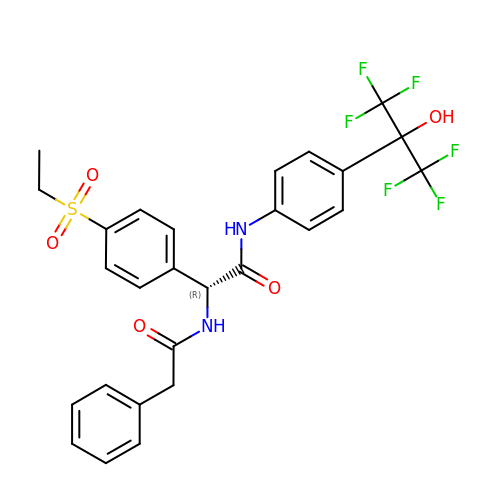(2~{R})-2-(4-ethylsulfonylphenyl)-~{N}-[4-[1,1,1,3,3,3-hexakis(fluoranyl)-2-oxidanyl-propan-2-yl]phenyl]-2-(2-phenylethanoylamino)ethanamide | C27 H24 F6 N2 O5 S | YNDQSYNAWXKDSD-HSZRJFAPSA-N> PQISRQEYAGLFGPTTGDKIRLGDTNLFIEIEKDLRGYGEESVYGGGKSLRDGMGANNHLTRDNGVLDLVITNVTIVDARLGVIKADVGIRDGKIAGIGKSGNPGVMDGVTPGLVVGVSTDAISGEHLILTAAGIDTHIHLISPQQAYHALSNGVATFFGGGIGPTDGTNGTTVTPGPWNIRQMLRSVEGLPVNVGILGKGNSYGRGPLLEQAIAGVVGYKVHEDWGATANALRHSLRMADEMDIQVSVHTDSLNECGYVEDTIDAFEGRTIHTFHTEGAGGGHAPDIIRVASQPNVLPSSTNPTLPYGVNSQAELFDMIMVCHNLNPNVPADVSFAESRVRPETIAAENVLHDMGVISMFSSDSQAMGRVGENWLRVMQTANAMKASRGKLPEDAPGNDNFRVLRYVAKITINPAIAQGVSHVIGSVEVGKMADLVLWDPRFFGAKPKMVIKGGMINWAAMGDPNASLPTPQPVFYRPMFGAM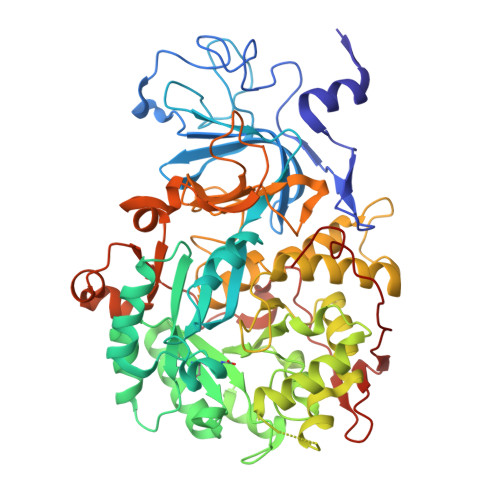GKTMQDTCVTFVSQAALDDGVKEKAGLDRQVIAVKNCRTISKHDLVRNDQTPNIEVDPETFAVKVDGVHATCEPIDTAAMNQRYFFG>MAANKSKGQSSLALHKVIMVGSGGVGKSALTLQFMYDEFVEDYEPTKADSYRKKVVLDGEEVQIDILDTAGLEDYAAIRDNYFRSGEGFLLVFSITEHESFTATAEFREQILRVKAEEDKIPLLVVGNKSDLEERRQVPVEEARSKAEEWGVQYVETSAKTRANVDKVFFDLMREIRTKKMSENK[2x];>GPLGSETQAGIKEEIRRQEFLLNSLHRDLQGGIKDLSKESRMWEVLRI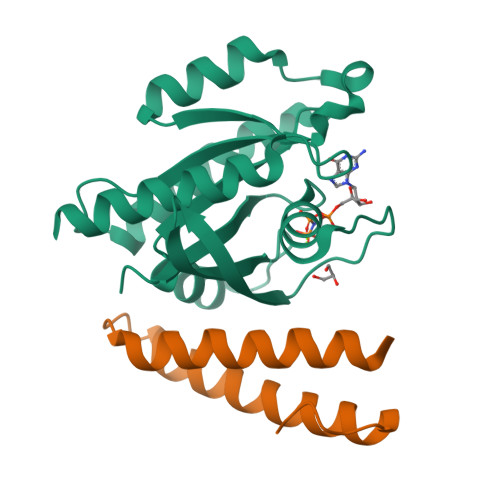LTALRRKLREA[2x]(1R,4R,6S)-1-methyl-4-(prop-1-en-2-yl)-7-oxabicyclo[4.1.0]heptane | 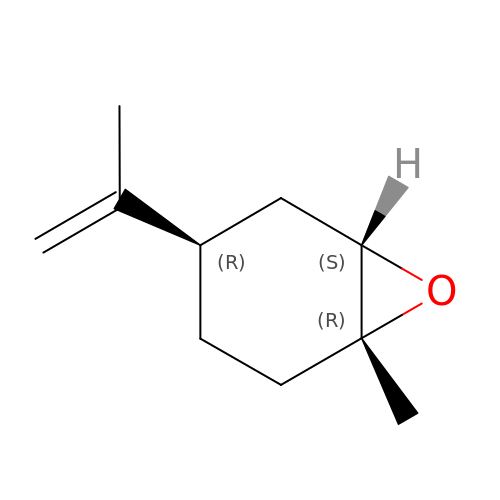C10 H16 O | CCEFMUBVSUDRLG-KXUCPTDWSA-N>[2x]SL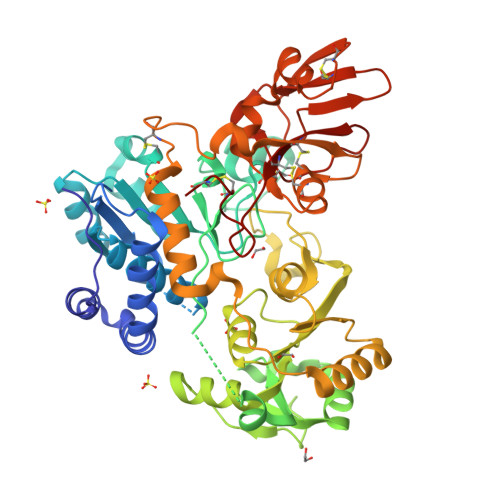AEIRTDFNILYSMMKKHEEFRWMRLRIRRMADAWIQAIKSLAEKQNLEKRKRKKVLVHLGLLTKESGFKIAETAFSGGPLGELVQWSDLITSLYLLGHDIRISASLAELKEIMGGGGVELIYIDIVGLAQFKKTLGPSWVHYQCMLRVLDSFGTEPEFNHANYAQSKGHKTPWGKWNLNPQQFYTMFPHTPDNSFLGFVVEQHLNSSDIHHINEIKRQNQSLVYGKVDSFWKNKKIYLDIIHTYMEVHATVYGSSTKNIPSYVKNHGILSGRDLQFLLRETKLFVGLGFPYEGPAPLEAIANGCAFLNPKFNPPKSSKNTDFFIGKPTLRELTSQHPYAEVFIGRPHVWTVDLNNQEEVEDAVKAILNQKIEPYMPYEFTCEGMLQRINAFIEKQDFCHGQVMWPPLSALQVKLAEPGQSCKQVCQESQLICEPSFFQHLNKDKDMLKYKVTCQSSELAKDILVPSFDPKNKHCVFQGDLLLFSCAGAHPRHQRVCPCRDFIKGQVALCKDCL>[4x]MTETSGTFNDIEARLAAVLEEAFEAGTSIYNERGFKRRIGYGNRPAVIHIDLANAWTQPGHPFSCPGMETIIPNVQRINEAARAKGVPVFYTTNVYRNRDASSGTNDMGLWYSKIPTETLPADSYWAQIDDRIAPADGEVVIEKNRAS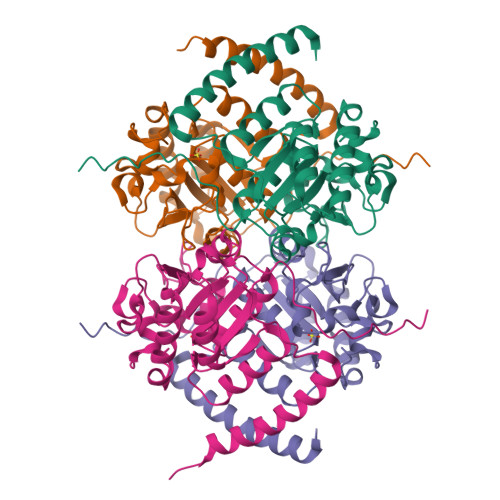AFPGTNLELFLTSNRIDTLIVTGATAAGCVRHTVEDAIAKGFRPIIPRETIGDRVPGVVQWNLYDIDNKFGDVESTDSVVQYLDALPQFEDTVPKTLSDPQPEVEAPADPVFAEQH> MGSSHHHHHHSQGSMSQDFVTLVSKDDKEYEISRSAAMISPTLKAGRIELKQFDSHILE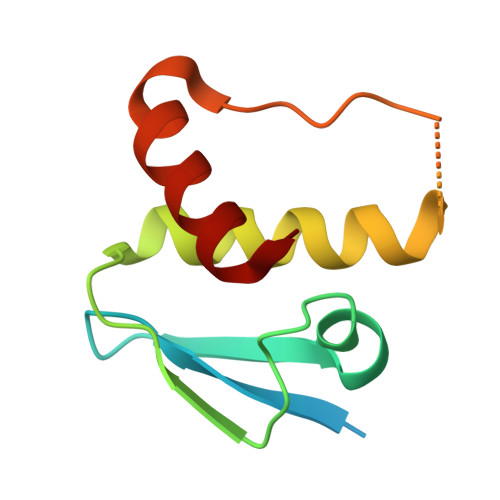KAVEYLNYNLKYSGVSEDDDEIPEFEIPTEMSLELLLAADYLSI> ILPDSVDWREKGCVTEVKYQGSCGASWAFSAVGALEAQLKLKTGKLVSLSAQNLVDCSTEKYGNKGCNGGFMTTAFQYIIDNKGIDSDASYPYKAMDQKCQYDSKYRAATCSKYTELPYGREDVLKEAVANKGPVSVGVDARHPSFFLYRSGVYYEPSCTQNVNHGVLVVGYGDLNGKEYWLVKNSWGHNFGEEGYIRMA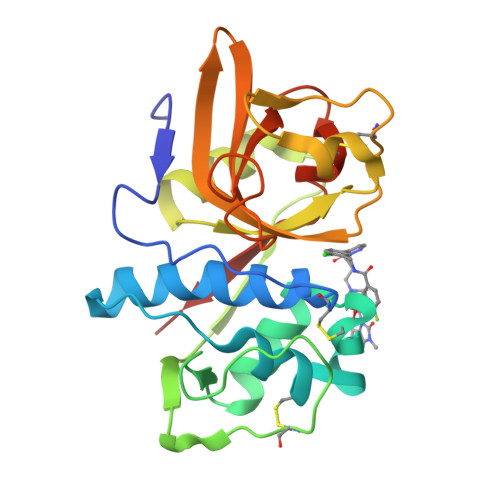RNKGNHCGIASFPSYPEILQGGG> MQAAALLLLVLRAITSIEAAADDVNPDDNKEDFAVLCALAALANLQTTVPSIDTSGLAAYDNLQQLNLSLSSKEWKSLFNKAADSNGSPKQPPEGFQSDPTWRKQWPIWVTAAAALKAENKEAAVLARAGLTNAPEELRNRARLALIPLLAQAEQIRDRLSEIQKQNEDTTPTAIAKALNKAVYGQDKETGAVYNSADCFSGNVADSTQNSCKAGNQASKATTVAATIVCVCHKKNGGNDAANACGRLINHQSDAGANLATASSDFGDIIATCAARPPKPLTAAYLDSALAAVSARIRFKNGNGYLGKFKATGCTGSASEGLCVEYTALTAATMQNFYKIPWVKEISNVAEALKRTEKDAAESTLLSTWLKASENQGNSVAQKLIKVGDSKAVPPAQRQTQNKPGSNCNKNLKKSECKDSDGCKWNRTEETEGDFCKPKET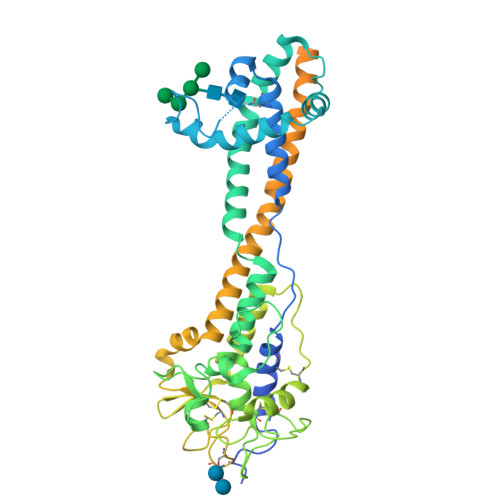GTENPAAGTGEGAAGANTETKKCSDKKTEGDCKDGCKWDGKECKDSSILATKKFALTVVSAAFVALLF> LGRLVSPGPCPRPYLVITEQPKQRGMRFRYECEGRSAGSILGESSTEASKTQPAIELRDCGGLREVEVTACLVWKDWPHRVHPHSLVGKDCTDGVCRVRLRPHVSPRHSFNNLGIQCVRKKEIEAAIERKIQLGIDPYNAGSLKNHQEVDMNVVRICFQASYRDQQGHLHRMDPILSEPVYDKKSTNTSELRICRINKESGPCTGGEELYLLCDKVQKEDISVVFSTASWEGRADFSQADVHRQIAIVFKTPPYEDLEISEPVTVNVFLQRLTDGVCSEPLPFTYLPR;> DGPYLQILEQPKQRGFRFRYVCEGPSHGGLPGASSEKNKKSYPQVKICNYVGPAKVIVQLVTNGKNIHLHAHSLVGKHCEDGVCTVTAGPKDMVVGFANLGILHVTKKKVFETLEARMTEACIRGYNPGLLVHSDLAYLQAEGGGDRQLTDREKEIIRQAAVQQTKEMDLSVVRLMFTAFLPDSTGSFTRRLEPVVSDAIYDSKAPNASNLKIVRMDRTAGCVTGGEEIYLLCDKVQKDDIQIRFYEEEEN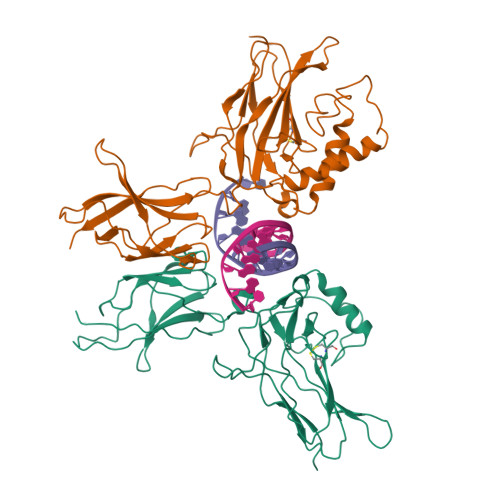GGVWEGFGDFSPTDVHRQFAIVFKTPKYKDVNITKPASVFVQLRRKSDLETSEPKPFLYYPEIKDKEEVQRKRQK> MQRCDWVSQDPLYIAYHDNEWGVPETDSRKLFEMICLEGQQAGLSWITV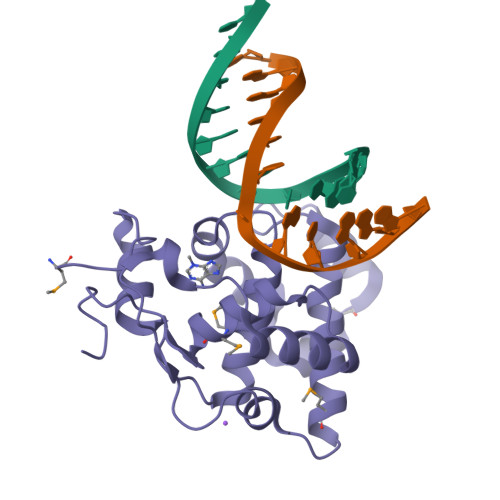LKKRENYRACFHQFDPIRIAAMQEEDVERLLQNTGIIRHRGKIQAIISNARAWLAMEQNGESFADFVWSFVDGQPQITQAASLDKIPTSTPASDALAKALKKRGFKFVGTTICYSFMQACGLVNDHITGCFCHPG(4S,7Z)-7-(2-amino-1,3-thiazol-4-yl)-1-[({4-[(2R)-2,3-dihydroxypropyl]-3-(4,5-dihydroxypyridin-2-yl)-5-oxo-4,5-dihydro-1H-1,2,4-triazol-1-yl}sulfonyl)amino]-4-formyl-10,10-dimethyl-1,6-dioxo-9-oxa-2,5,8-triazaundec-7-en-11-oate | C23 H27 N10 O13 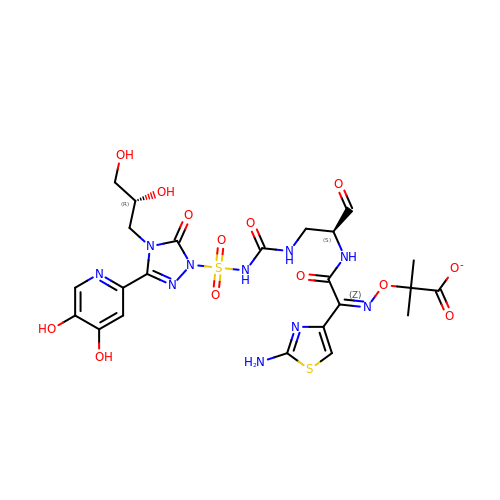S2 | CVHWOSQJHWFYSJ-DXKYJFGHSA-M> MEDKGKTFFGQPLGLSTLFMTEMWERFSYYGMRAILLYYMWFLISTGDLHITRATAASIMAIYASMVYLSGTIGGFVADRIIGARPAVFWGGVLIMLGHIVLALPFGASALFGSIILIIIGTGFLKPNVSTLVGTLYDEHDRRRDAGFSIFVFGINLGAFIAPLIVGAAQEAAGYHVAFSLAAIGMFIGLLVYYFGGKKTLDPHYLRPTDPLAPEEVKPLLVKVSLAVAGFIAIIVVMNLVGWNSLPAYINLLTIVAIAIPVFYFAWMISSVKVTSTEHLRVVSYIPLFIAAVLFWAIEEQGSVVLATFAAERVDSSWFPVSWFQSLNPLFIMLYTPFFAWLWTAWKKNQPSSPTKFAVGLMFAGLSFLLMAIPGALYGTSGKVSPLWLVGSWALVILGEMLISPVGLSVTTKLAPKAFNSQMMSMWFLSSSVGSALNAQLVTLYNAKSEVAYFSYFGLGSVVLGIVLVFLSKRIQGLMQGVEAENLYFQ

Proton-dependent oligopeptide transporters (POTs; also known by the acronyms PepTs and PTRs) are ubiquitous in bacteria and eukaryotes where they play an important role in nitrogen acquisition through proton-coupled uptake of di- and tripeptides (Daniel et al., 2006, Smith et al., 2013). POTs belong to the major facilitator superfamily (MFS), and therefore adopt a canonical MFS fold where two 6-helical MFS domains, the N domain and the C domain, cradle a centrally located substrate binding cavity (Quistgaard et al., 2016, Yan, 2015). The MFS fold enables substrate transport through an alternating access mechanism, which involves conformational transitions between inward open, outward open, and occluded states (Newstead, 2015, Quistgaard et al., 2016, Yan, 2015). Twenty-eight peptides were screened for binding to PepTSt from Streptococcus thermophilus, and structures were determined of PepTSt in complex with four physicochemically diverse dipeptides, which bind with millimolar affinity: Ala-Leu, Phe-Ala, Ala-Gln, and Asp-Glu.

Furthermore, Ala-Gln was also found to bind well, implying that a glutamine residue can be accommodated in the second position. The structures of PepTSt were determined in complex with four dipeptides that collectively represent substantial sequence variation: Ala-Leu, Phe-Ala, Ala-Gln, and Asp-Glu. These peptides, furthermore, bind with a rather wide range of affinities: high in the case of Ala-Leu (0.56 mM), intermediate for Ala-Gln (6.82 mM) and Phe-Ala (10.95 mM), and rather weak for Asp-Glu (>50 mM). The structures were refined to maximum resolutions of 2.7–2.2 Å, and were either in the inward open conformation (PepTSt[Phe-Ala], PepTSt[Asp-Glu]) or in an inward-facing partially occluded form (PepTSt[Ala-Leu], PepTSt[Ala-Gln]), which mainly differs from the former by exhibiting pronounced bending of transmembrane helices 10 and 11 (TM10 and TM11) (Lyons et al., 2014, Quistgaard et al., 2017). An overlay of the structures reveals that the peptide backbones of Ala-Phe, Ala-Leu, Ala-Gln, and Asp-Glu overlap strongly with each other, while Phe-Ala adopts a markedly different position. The backbone interactions of Ala-Leu, Ala-Gln, and Asp-Glu are similar to those previously described for Ala-Phe (Lyons et al., 2014): The N-terminal residue interacts with Asn-156, Glu-299, Asn-328, and Glu-400, while the C-terminal residue interacts with Arg-26, Tyr-30, and Lys-126. Ala-Gln binds in much the same position as Ala-Leu. Yet the glutamine side chain is bound quite differently than leucine: Tyr-68 and to a lesser extent Trp-296 have moved closer to it, thus narrowing the pocket around it and enabling the formation of van der Waals interactions as well as a putative N-H···π bond mediated by Trp-296. In addition, Trp-427 and Ser-431 have undergone rotameric shifts in order to form hydrogen bonds to the side-chain amide.>MGHHHHHHKKPLKKGRANKKNDRDSPSSTFVDWNGPCLRLQYPLFDIEYLRSHEIYSGTPIQSISLRTNSPQPTSLTSDNDTSSVTTAKLQSILFSNYMEEYKVDFKRSTAIYNPMSEIGKLIEYSCLVFLPSPYAEQLKETILPDLNASFDNSDTKGFVNAINLYNKMIREIPRQRIIDHLETIDKIPRSFIHDFLHIVYTRSIHPQANKLKHYKAFSNYVYGELLPNFLSDVYQQCQLKKGDTFMDLGSGVGNCV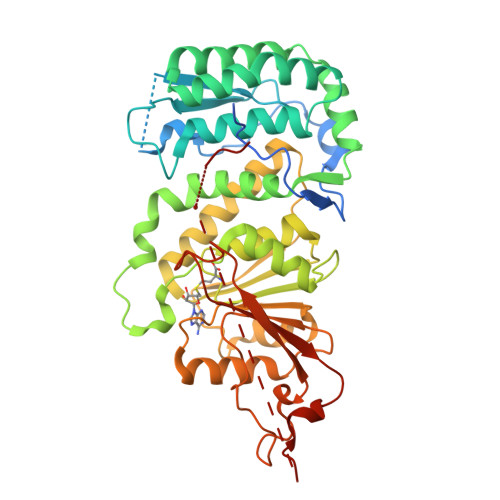VQAALECGCALSFGCEIMDDASDLTILQYEELKKRCKLYGMRLNNVEFSLKKSFVDNNRVAELIPQCDVILVNNFLFDEDLNKKVEKILQTAKVGCKIISLKSLRSLTYQINFYNVENIFNRLKVQRYDLKEDSVSWTHSGGEYYISTVMEDVDESLFSPAARGRRNRGTPVKYTR[3x]>MSHAHKKHKENAPKSLNFYVITISTSRYEKLLKKEPIVDESGDIIKQLLIENGHKIIGYSLVPDDKIKILKAFTDALSID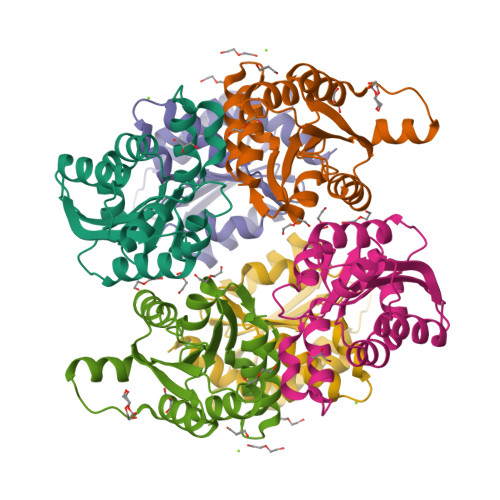EVDVIISTGGTGYSPTDITVETIRKLFDREIEGFSDVFRLVSFNDPEVKAAAYLTKASAGIIGKKIVYLLPGSPDAVKLALKELILPEVGHLVYLVRS[3x]BAP29 and BAP31 are two homologous membrane proteins (∼50% sequence identity in humans) that reside in the endoplasmic reticulum (ER). They both consist of an N-terminal membrane-bound domain with three predicted transmembrane helices, and a C-terminal cytoplasmic region, which encompass ∼50% of the protein and is predicted to form a coiled coil, or more likely two coiled coils. BAP31 controls the fates of its bound clients, which may be either retained in the ER, progress through the secretory pathway or be extruded and subjected to ER-associated degradation. The structures presented here now show for the first time that the vDED domain adopts a dimeric coiled coil fold with no structural similarity to DED domains.

The structure of the vDED domain of BAP31 was determined in two different crystal forms; P21 at pH 8.0 and twinned P3221 at pH 4.2. The vDED domain forms an uninterrupted parallel coiled coil dimer in both structures. Almost all residues could be modeled in the P21 form (172–233), but not in the P3221 form (169–220). Apart from that, the two structures are however quite similar and exhibit a RMSD Cα value of 1.12 Å for 94 aligned residues. It is surprising that part of the structure was disordered at pH 4.2, as the CD experiments show that the domain is considerably more stable at this pH than at neutral pH. We have no obvious explanation for this observation, but one possibility is that certain buffer molecules in the crystallization condition e.g. LiSO4 lead to partial unwinding of the coiled coil. In contrast, BAP31 vDED forms a coiled coil over a wide pH spectrum although the melting temperature is 11 °C higher at pH 4.2 than at pH 7.0. This dramatic increase in stability is puzzling since there is no clear evidence for any substantial charge repulsion in the dimer interface at pH 7.0 (though Glu-174 may perhaps cause some level of repulsion), and since very low pH may in fact destabilize the 2–3 inter-helical salt bridges that are present in the domain through protonation of acidic residues. However, several cases have been reported of coiled coils being stabilized at highly acidic pH in spite of a loss of salt bridges. A possible explanation for this is that the loss of ionic interactions at acidic pH may be counteracted by favorable interactions between basic residues and anions present in the solvent, reminiscent of the counterion condensation observed in double stranded DNA.

>[2x]SMLDVGNAEVKLEEENRSLKADLQKLKDELASTKQKLEKAENQVLAMRKQSEGLTKEYDRLLEEHAKL> MSSRNNPARVAIVMGSKSDWATMQFAAEIFEILNVPHHVEVVSAQRTPDKLFSFAESAEENGYQVIIAGAGGAAHLPGMIAAKTLVPVLGVPVQSAALSGVDSLYSIVQMPRGIPVGTLAIGKAGAANAALLAAQILATHDKELHQRLNDWRKA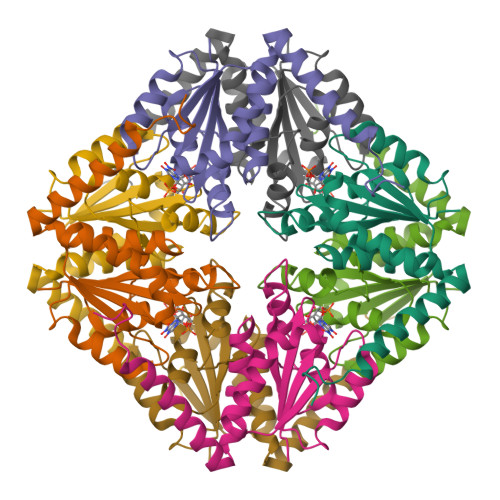QTDEVLENPDPRGAA> MRQSDPKVQVYSRNPGEYGKANVLIC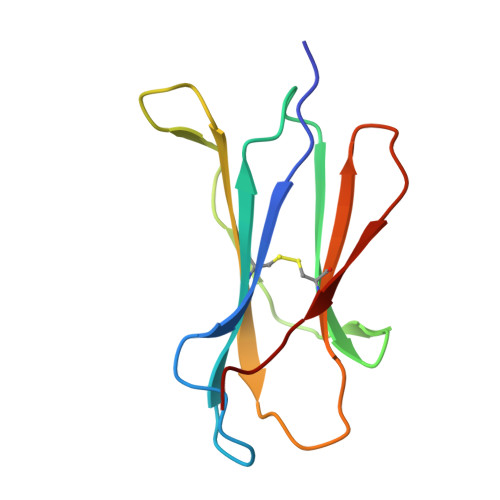YVSGFHPPDITIQLLKNGVEIPGSTQTDLAFEEGWQFHLTKYVDFLPQPGEEYTCRVRHMSSPTKSYTWEPDM> MALRGTVTDFSGFDGRADAEVLRKAMKGLGTDEDSILNLLTARSNAQRQQIAEEFKTLFGRDLVNDMKSELKGKFEKLIVALMKPSRLYDAYELKHALKGAGTDEKVLTEIIASRTPEELRAIKQAYEEEYGSNLEDDVVGDTKGYYQRMLVVLLQANRDPDTAIDDAQVELDAQALFQAGE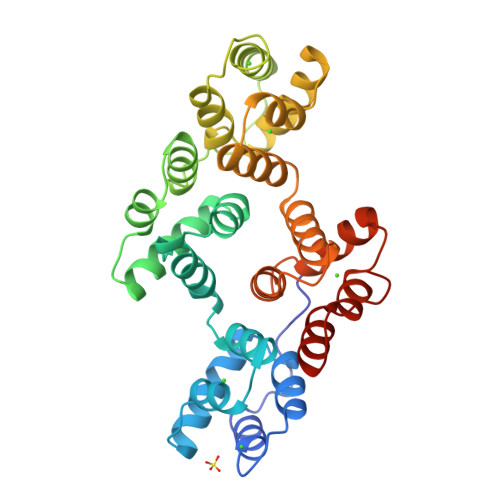LKWGTDEEKFITILGTRSVSHLRRVFDKYMTISGFQIEETIDRETKGNLENLLLAVVKSIRSIPAYLAETLYYAMKGAGTDDHTLIRVIVSRSEIDLFNIRKEFRKNFATSLYSMIKGDTKGDYKKALLLLCGGEDD> MKLKGEAVLITGGASGLGRALVDRFVAEGAKVAVLDKSAERLAELETDHGDNVLGIVGDVRSLEDQKQAASRCVARFGKIDTLIPNAGIWDYSTALVDLPEESLDAAFDEVFHINVKGYIHAVKACLPALVASRGNVIFTISNAGFYPNGGGPLYTAAKHAIVGLV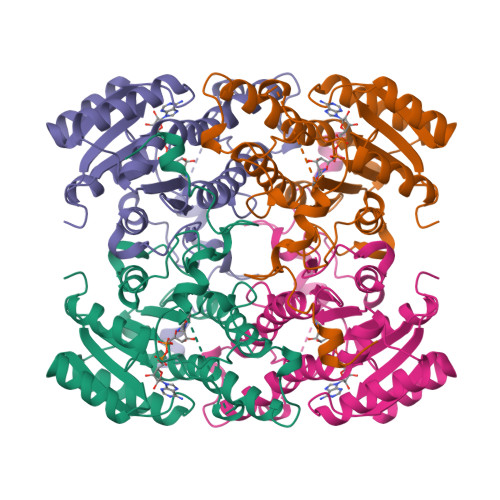RELAFELAPYVRVNGVGSGGINSDLRGPSSLGMGSKAISTVPLADMLKSVLPIGRMPEVEEYTGAYVFFATRGDAAPATGALLNYDGGLGVRGFFSGAGGNDLLEQLNIHP>MAASGEARRVLVYGGRGALGSRCVQAFRARNWWVASIDVVENEEASASVIVKMTDSFTEQADQVTAEVGKLLGDQKVDAILCVAGGWAGGNAKSKSLFKNCDLMWKQSIWTSTISSHLATKHLKEGGLLTLAGAKAALDGTPGMIGYGMAKGAVHQLCQSLAGKNSGMPSGAAAIAVLPVTLDTPMN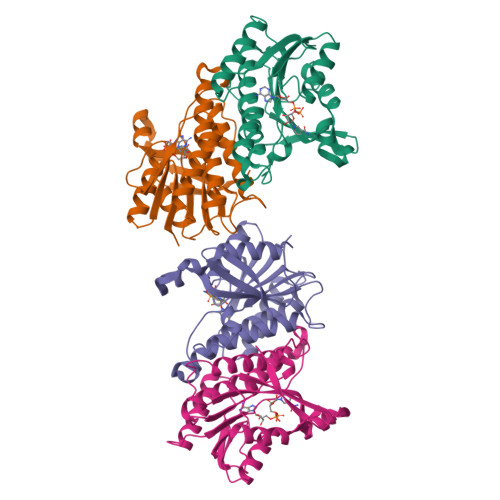RKSMPEADFSSWTPLEFLVETFHDWITGNKRPNSGSLIQVVTTDGKTELTPAYF[4x]The tip of each stereocilium is linked to its tallest neighbor by a ‘tip link' filament essential for hair-cell mechanotransduction. Immature tip links are likely formed by homotetrameric protocadherin-15 (PCDH15) proteins, while mature tip links are made of cadherin-23 (CDH23) and PCDH15 heterotetramers. CDH23 and PCDH15 are unusual members of the family that feature 27 and 11 EC repeats, respectively. Here we present the X-ray crystal structures of repeats EC8–10 and EC9–10 refined at 2.8 and 3.35 Å resolution, respectively, which show an EC9–10 calcium-free linker that alters the linear arrangement of PCDH15's EC repeats.

The solved structure of the human PCDH15 EC8–10 (2.8 Å) contained 333 residues starting from Ser 795 (EC8) to Glu 1,125 (numbering corresponds to the processed protein) followed by two histidine residues that are part of the purification tag. Overall, each of the three EC repeats shows an architecture similar to that of classical cadherins, with the typical Greek-key motif comprised of seven β strands forming a β sandwich fold. In addition, repeats EC8 and EC9 feature an α-helix between β strands C and D, also observed in some of the CDH23 and PCDH15 EC1–2 repeats. The first unique structural feature of PCDH15 EC8–10 is a canonical-like calcium-binding site at the EC8–9 linker with a novel torsion between these EC repeats. As expected, the structure shows three bound calcium ions. However, a comparison with PCDH15 EC1–2 and other cadherins reveals that the distance between calcium ions at positions 2 and 3 is larger in PCDH15 EC8–9 (8.48 Å versus an average of 6.84 Å for 41 canonical linkers). In PCDH15 EC8–9, the side chain of Asp 933 in the DXD motif, which usually bridges calcium ions at sites 2 and 3, only coordinates calcium at site 3 in a ‘canonical-like' architecture. The canonical DXNDN linker motif is DMNDY (897–901) in PCDH15 EC8–9, with the carbonyl oxygen of Tyr 901 coordinating calcium. It is likely that the bulky and conserved side chain of Tyr 901 and two proline residues after the DXD motif in EC9 (934–935; also conserved, Supplementary Fig. 4) cause the bending and atypical separation observed between ions at sites 2 and 3. In addition, the EC9–10 linker is calcium-free and bent (90°), with an EC9–10 310 helix and an EC10 FG-α loop that define the EC9–10 interface. Overall, these results indicate that the PCDH15 EC8–10 crystallographic conformation, including bending at EC9–10, is also observed in solution.

> MSPVFTNSTYTVLVEENLPAGTTILQIEAKDVDLGANVSYRIRSPEVKHFFALHPFTGELSLLRSLDYEAFPDQEASITFLVEAFDIYGTMPPGIATVTVIVKDMNDYPPVFSKRIYKGMVAPDAVKGTPITTVYAEDADPPGLPASRVRYRVDDVQFPYPASIFEVEEDSGRVITRVNLNEEPTTIFKLVVVAFDDGEPVMSSSATVKILVLHPGEIPRFTQEEYRPPPVSELATKGTMVGVISAAAINQSIVYSIVSGNEEDTFGINNITGVIYVNGPLDYETRTSYVLRVQADSLEVVLANLRVPSKSNTAKVYIEIQDENNHPPVFLEHHHHHH> ADIFDSFELLYDRPGEPMINTKGEDKVLFELTEQFLTPEYANNGLELNNRFGDEEEVSRKIILKNLDKIPEFPKAKQLPNDADFSLFLPSHQEMANEVIDVLMSVTENQLQELLSTCVYARINLNPQLFNYCYTVAIMHRRDTGKVRVQNYAEIFPAKFLDSQVFTQAREAAAVIPKTIPRTPIIIPRDYTATDLEEEHRLAYWREDLGINLHHWHWHLVYPFSASDEKIVAKDRRGELFFYMHQQIIARYNCERLCNSLKRVKKFSDWREPIPEAYYPKLDSLTSARGWPPRQAGMRWQDLKRPVDGLNVTIDDMERYRRNIEEAIATGNVILPDKSTKKLDIDMLGNMMEASVLSPNRDLYGSIHNNMHSFSAYMHDPEHRYLESFGVIADEATTMRDPFFYRVHAWVDDIFQSFKEAPHNVRPYSRSQLENPGVQVTSVAVESAGGQQNVLNTFWMQSDVNLSKGLDFSDRGPVYARFTHLNHRPFRYVIKANNTASARRTTVRIFIAPKTDERNLPWALSDQRKMFIEMDRFVVPLSAGENTITRQSTESSLTIPFEQTFRDLSIQGSDPRRSELAAFNYCGCGWPQHMLVPKGTVGGVAYQLFVMLSNYELDKIEQPDGRELSC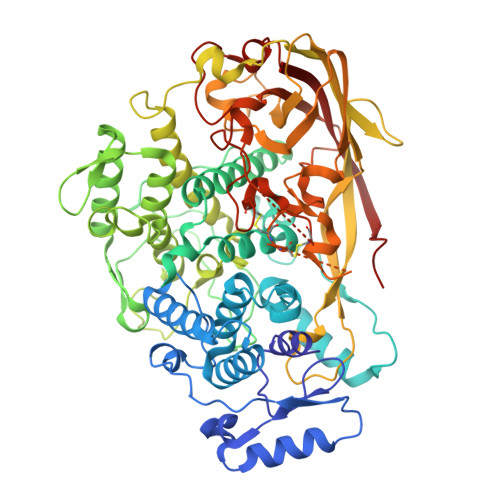VEASMFCGLKDKKYPDARPMGYPFDRPSNSATNIEDFSAMSNMGLQDIVIKLSDVTEPNPRNPPA>[2x]MICSVTGKPVKDVLSTFFKDRNDVLESEVKKFHLLATFEECKALAADTARRMNEYYKDVAEPVTLVALLTGAYLYASLLTVHLTFPYTLHFVKVS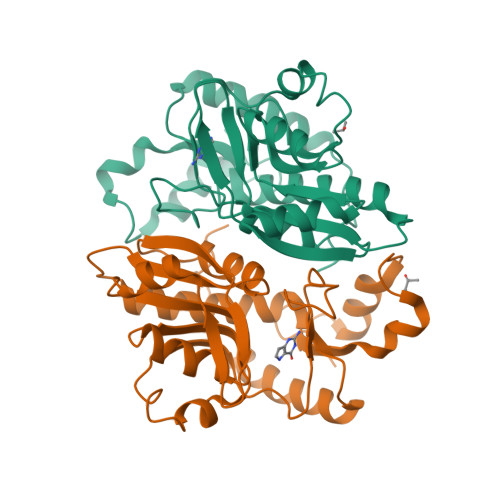SYKGTRQESVVFDEEDLKQLKEKREVVLIDEYVDSGHTIFSIQEQIKHAKICSCFVKDVDAIKKHSALADTKMFYGYTPMPKGSWLIGFGLDDNGLRRGWAHLFDINLSESEVTEFRRRLTEHIKGLNINGVNRY>MILGIDIGGANTKITELHENGEFKVHHLYFPMWKNNDKLAEVLKTYSNDVSHVALVTTAELADSYETKKEGVDNILNAAESAFGSNISVFDSNGNFISLESAKTNNMKVSASNWCGTAKWVSKNIEENCILVDMGSTTTDIIPIVEGKVVAEKTDLERLMNHELLYVGTLRTPISHLGNTISFKGVDTNVSSEYFAITADISVVLEKVTTEEYTCDTPDGKGTD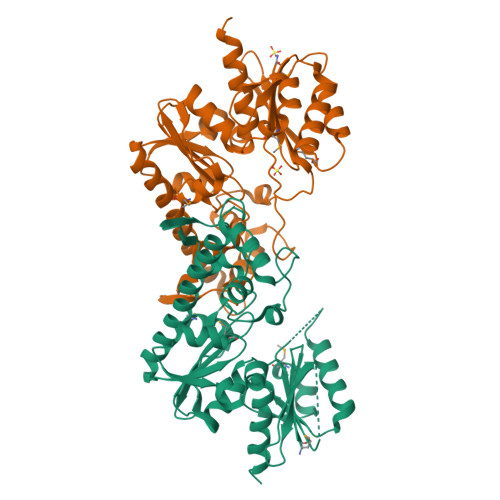KRSSLVRISKVLCSDLDQISEIDAENIAKNYYELWKELILENVENVAEKYGSKKVVITGLGENILKDALADFEVISVAERYGKDVSLATPSFAVAELLKNELLEHHHHHH[2x]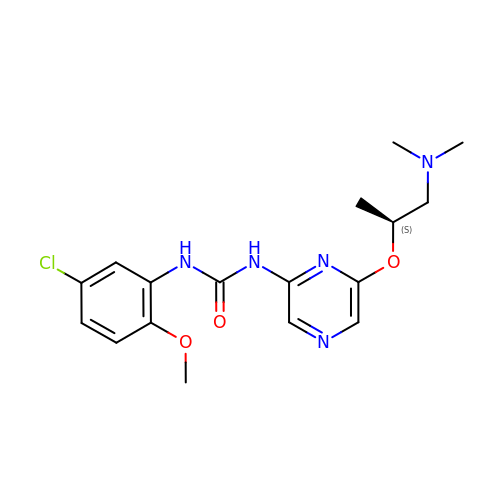1-(5-CHLORO-2-METHOXYPHENYL)-3-{6-[2-(DIMETHYLAMINO)-1-METHYLETHOXY]PYRAZIN-2-YL}UREA | C17 H22 Cl N5 O3 | GIAYFZLMPSVQDV-NSHDSACASA-N>[3x]MNLVNKAQLQKMAYVKFRIQEDEYVAILNALEEYHNMSESSVVEKYLKLKDINNLTDNYLNTYKKSGRNKALKKFKEYLTMEVLELKNNSLTPVEKNLHFIWIGGQINDTAINYINQWKDVNSDYTVKVFYDSNAFLINTLKKTIVESATNNTLESFRENLNDPEFDYNKFYRKRMEIIYDKQKHFIDYYKSQIEENPEFIIDNIIKTYLSNEYSKDLEALNKYIEESLNKITANNGNDIRNLEKFADEDLVRLYNQELVERWNLAAASDILRISMLKEDGGVYLDVDMLPGIQPDLFKSINKPDSITNTSWEMIKLEAIMKYKEYIPGYTSKNFDMLDEEVQRSFESALSSKSDKSEIFLPLDDIKVSPLEVKIAFANNSVINQALISLKDSYCSDLVINQIKNRYKILNDNLNPSINEGTDFNTTMKIFSDKLASISNEDNMMFMIKITN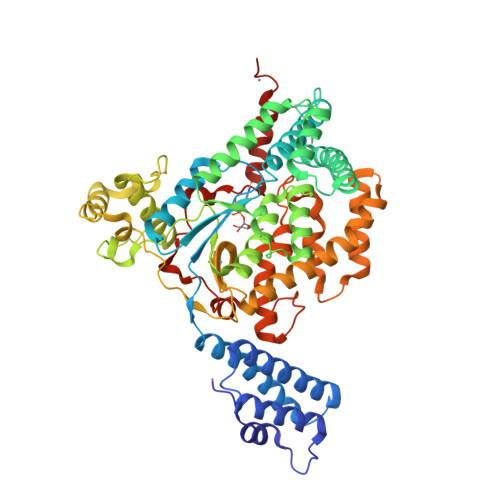YLKVGFAPDVRSTINLSGPGVYTGAYQDLLMFKDNSTNIHLLEPELRNFEFPKTKISQLTEQEITSLWSFNQARAKSQFEEYKKGYFEGALGED[(1S)-1-{[6-(4-methylphenyl)thieno[2,3-d]pyrimidin-4-yl]amino}-2-phenylethyl]phosphonic acid | C21 H20 N3 O3 P S | 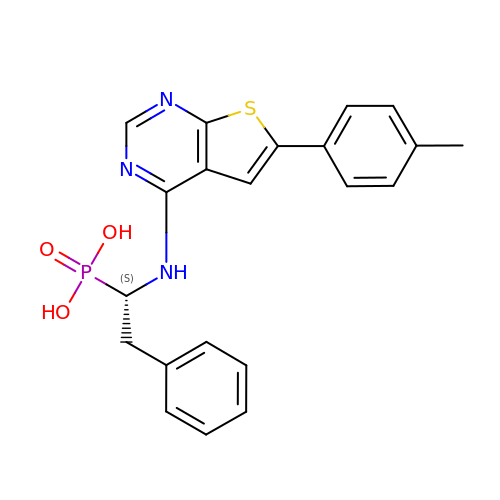UYKRLVOVLULTHW-IBGZPJMESA-N>[2x]DNDPLVVNTDKGRIRGITVDAPSGKKVDVWLGIPYAQPPVGPLRFRHPRPAEKWTGVLNTTTPPNSCVQIVDTVFGDFPGATMWNPNTPLSEDCLYINVVAPRPRPKNAAVMLWIFGGGFYSGTATLDVYDH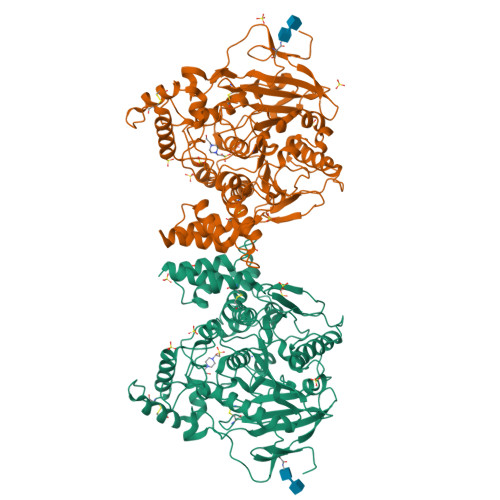RALASEENVIVVSLQYRVASLGFLFLGTPEAPGNAGLFDQNLALRWVRDNIHRFGGDPSRVTLFGESAGAVSVSLHLLSALSRDLFQRAILQSGSPTAPWALVSREEATLRALRLAEAVGCPHEPSKLSDAVECLRGKDPHVLVNNEWGTLGICEFPFVPVVDGAFLDETPQRSLASGRFKKTEILTGSNTEEGYYFIIYYLTELLRKEEGVTVTREEFLQAVRELNPYVNGAARQAIVFEYTDWTEPDNPNSNRDALDKMVGDYHFTCNVNEFAQRYAEEGNNVYMYLYTHRSKGNPWPRWTGVMHGDEINYVFGEPLNPTLGYTEDEKDFSRKIMRYWSNFAKTGNPNPNTASSEFPEWPKHTAHGRHYLELGLNTSFVGRGPRLRQCAFWKKYLPQLVAATSNLPGPAPPSEPCESSA>[8x]MGHHHHHHMVLMTKPGTSDFVWNGIPLSMELNLWNIKEYSGSVAMKFDGEKITFDADIQ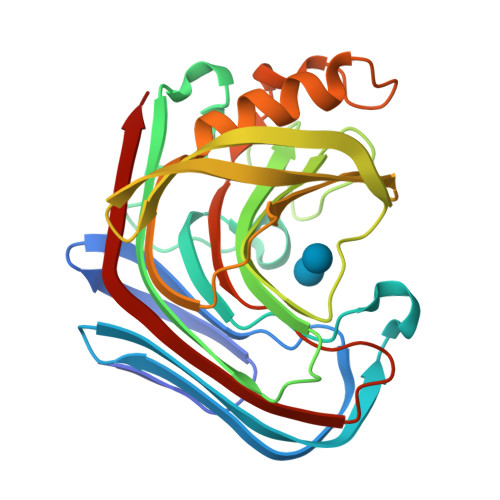NLSPKEPERGVLGYPEFYYGYKPWENHTAEGSKLPVPVSSMKSFSVEVSFDIHHEPSLPLNFAMETWLTREKYQTEASIGDVEIMVWFYFNNLTPGGEKIEEFTIPFVLNGESVEGTWELWLAEWGWDYLAFRLKDPVKKGRVKFDVRHFLDAAGKALSSSARVKDFEDLYFTVWEIGTEFGSPETKSAQFGWKFENFSIDLEVRE> VFPSSVYVPDEWEVSREKITLLRELGQGSFGMVYEGNARDIIKGEAETRVAVKTVNESASLRERIEFLNEASVMKGFTCHHVVRLLGVVSKGQPTLVVMELMA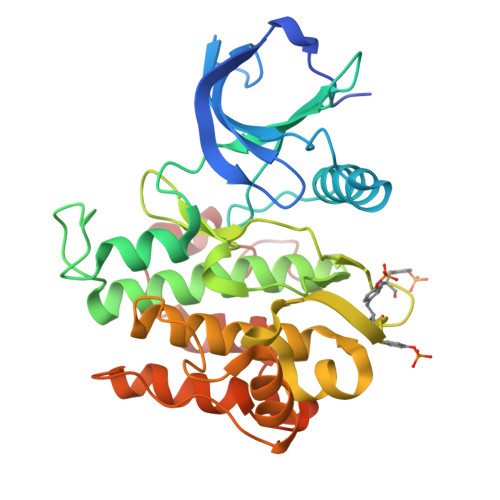HGDLKSYLRSLRPEAENNPGRPPPTLQEMIQMAAEIADGMAYLNAKKFVHRDLAARNCMVAHDFTVKIGDFGMTRDIYETDYYRKGGKGLLPVRWMAPESLKDGVFTTSSDMWSFGVVLWEITSLAEQPYQGLSNEQVLKFVMDGGYLDQPDNCPERVTDLMRMCWQFNPNMRPTFLEIVNLLKDDLHPSFPEVSFFHSEENK>MPMVLLECDKDIPERQKHIYLKAPNEDTREFLPIANAATIPGTLSERGCAFCGAKLVIGGVLKDTIQMIHGPLGCAYDTWHTKRYPTDNGHFNMKYVWSTDMKESHVVFGGEKRLEKSMHEAFDEMPDIKRMIVYTTCPTALIGDDIKAVAKKVMKDRPDVDVFT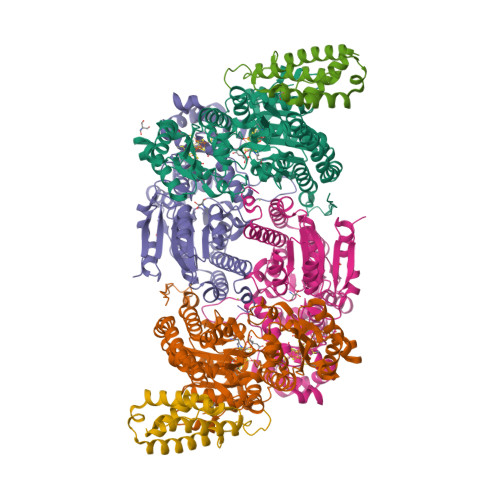VECPGFSGVSQSKGHHVLNIGWINEKVETMEKEITSEYTMNFIGDFNIQGDTQLLQTYWDRLGIQVVAHFTGNGTYDDLRCMHQAQLNVVNCARSSGYIANELKKRYGIPRLDIDSWGFNYMAEGIRKICAFFGIEEKGEELIAEEYAKWKPKLDWYKERLQGKKMAIWTGGPRLWHWTKSVEDDLGVQVVAMSSKFGHEEDFEKVIARGKEGTYYIDDGNELEFFEIIDLVKPDVIFTGPRVGELVKKLHIPYVNGHGYHNGPYMGFEGFVNLARDMYNAVHNPLRHLAAVDIRDKSQTTPVIVRGAA[2x];>MSNCELTVLKPAEVKLSPRDREGIINPMYDCQPAGAQYAGIGIKDCIPLVHGGQGCTMFVRLLFAQHFKENFDVASTSLHEESAVFGGAKRVEEGVLVLARRYPNLRVIPIITTCSTEVIGDDIEGSIRVCNRALEAEFPDRKIYLAPVHTPSFKGSHVTGYAECVKSVFKTITDAHGKGQPSGKLNVFPGWVNPGDVVLLKRYFKEMDVEANIYMDTEDFDSPMLPNKSIETHGRTTVEDIADSANALATLSLARYEGNTTGELLQKTFAVPNALVNTPYGIKNTDDMLRKIAEVTGKEIPESLVRERGIALDALADLAHMFFANKKVAIFGHPDLVLGLAQFCMEVELEPVLLLIGDDQGNKYKKDPRIEELKNTAHFDIEIVHNADLWELEKRINAGLQLDLIMGHSKGRYVAIEANIPMVRVGFPTFDRAGLYRKPSIGYQGAMELGEMIANAMFAHMEYTRNKEWILNTW[2x];>MSQSHLDDLFAYVEERCLWQFFSRTWDREENIEGVLNQVGRLLTGQEPLRGTPQERLFYADALAMANDVRERFPWASQVNKEEIEFLLDGLKSRLVDVTITRSTNRELNHHLY[2x]>[2x]MKLAYSLLLPLAGVSASVINYKRDGDSKAITNTTFSLNRPSVHFTPSHGWMNDPNGLWYDAKEEDWHLYYQYNPAATIWGTPLYWGHAVSKDLTSWTDYGASLGPGSDDAGAFSGSMVIDYNNTSGFFNSSVDPRQRAVAVWTLSKGPSQAQHISYSLDGGYTFQHYSDNAVLDINSSNFRDPKVFWHEGENGEDGRWIMAVAESQVFSVLFYSSPNLKNWTLESNFTHHGWTGTQYECPGLVKVPYDSVADSSSNSSDSKPDSAWVLFVSINPGGPLGGSVTQYFVGDFNGTHFTPIDDQTRFLDMGKDYYALQTFFNTPNEKDVYGIAWASNWQYAQQAPTDPWRSSMSLVRQFTLKDFSTNPNSADVVLNS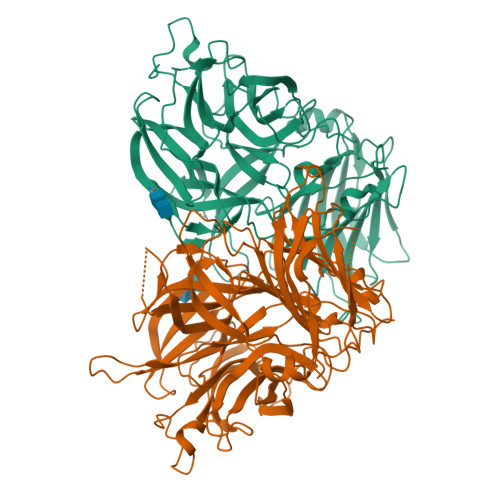QPVLNYDALRKNGTTYSITNYTVTSENGKKIKLDNPSGSLEFHLEYVFNGSPDIKSNVFADLSLYFKGNNDDNEYLRLGYETNGGAFFLDRGHTKIPFVKENLFFNHQLAVTNPVSNYTTNVFDVYGVIDKNIIELYFDNGNVVSTNTFFFSTNNVIGEIDIKSPYDKAYTINSFNVTQFNV>[6x]MKVLFLTANEFEDVELIYPYHRLKEEGHEVYIASFERGTITGKHGYSVKVDLTFDK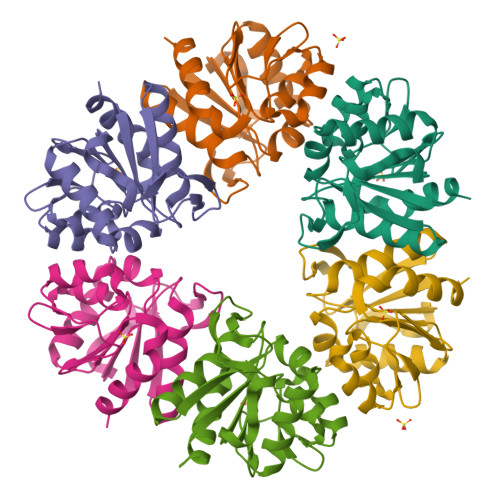VNPEEFDALVLPGGRAPERVRLNEKAVSIARKMFSEGKPVASICHGPQILISAGVLRGRKGTSYPGIKDDMINAGVEWVDAEVVVDGNWVSSRVPADLYAWMREFVKLLK> GSV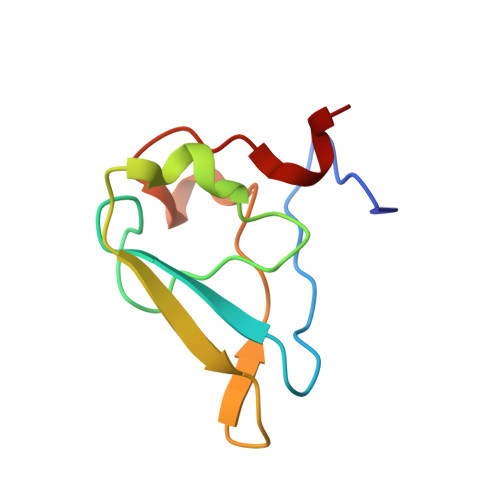HKHTGRNCGRKFKIGEPLYRCHECGCDDTCVLCIHCFNPKDHVNHHVCTDICTEFTSGICDCGDEEAWNSPLHCKAEEQ> MGNCLDSSAKVDNSNHSPHANSASSGSKVSSKTSRSTGPSGLSTTSYSTDSSFGPLPTLRTEGEILSSPNLKAFTFNELKNATKNFRQDNLLGEGGFGCVFKGWIDQTSLTASRPGSGIVVAVKQLKPEGFQGHKEWLTEVNYLGQLSHPNLVLLVGYCAEGENRLLVYEFMPKGSLENHLFRRGAQPLTWAIRMKVAVGAAKGLTFLHEAKSQVIYRDFKAANILLDADFNAKLSDFGLAKAGPTGDNTHVSTKVIGTHGYAAPEYVATGRLTAKSDVYSFGVVLLELI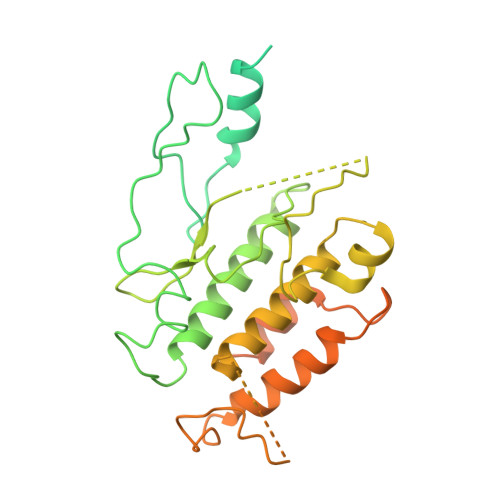SGRRAMDNSNGGNEYSLVDWATPYLGDKRKLFRIMDTKLGGQYPQKGAFTAANLALQCLNPDAKLRPKMSEVLVTLEQLESVAKPGTKHTQMESPRFHHSSVMQKSPVRYSHDRPLLHMTPGASPLPSYTQSPRVR>[4x]MGSSHHHHHHSSGLQGTENLYFQSHMTILVVTGTGTGVGKTVVCAALASAARQAGIDVAVCKPVQTGTARGDDDLAEVGRLAGVTQLAGLARYPQPMAPAAAAEHAGMALPARDQIVRLIADLDRPGRLTLVEGAGGLLVELAEPGVTLRDVAVDVAAAALVVVTADLGTLNHTKLTLEALAAQQVSCAGLVIGSWPDPPGLVAASNRSALARIAMVRAALPAGAASLDAGDFAAM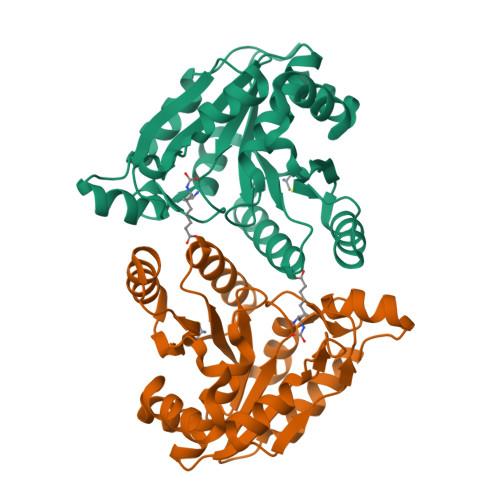SAAAFDRNWVAGLVG> GNSVTYNTL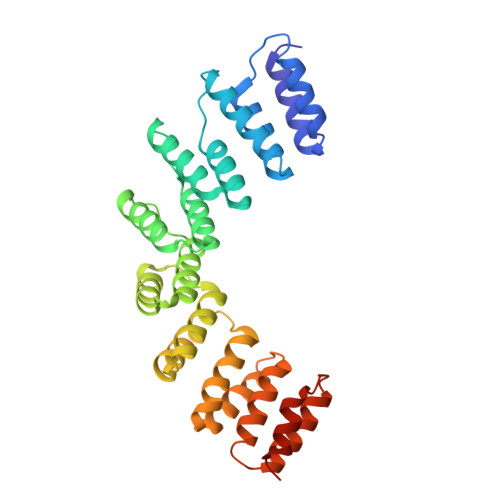ISGLGKAGRLEEALELFEEMKEKGIVPSVVTYNTLISGLGKAGRLEEALELFEEMKEKGIVPSVVTYNTLISGLGKAGRLEEALELFEEMKEKGIVPSVVTYNTLISGLGKAGRLEEALELFEEMKEKGIVPSVVTYNTLISGLGKAGRLEEALELFEEMKEKGIVPSVVTYNTLISGLGKAGRLEEALELFEEMKEKGIVPSVVTYNTLISGLGKAGRLEEALELFEEMKEKGIVPSVVTYNTLISGLGKAGRLEEALELFEEMKEKGIVPSVVTYNTLISGLGKAGCGRALE>MSQHNEKNPHQHQSPLHDSSEAKPGMDSLAPEDGSHRPAAEPTPPGAQPTAPGSLKAPDTRNEKLNSLEDVRKGSENYALTTNQGVRIADDQNSLRAGSRGPTLLEDFILREKITHFDHERIPERIVHARGSAAHGYFQPYKSLSDITKADFLSDPNKITPVFVRFSTVQGGAGSADTVRDIRGFATKFYTEEGIFDLVGNNTPIFFIQDAHKFPDFVHAVKPEPHWAIPQGQSAHDTFWDYVSLQPETLHNVMWAMSDRGIPRSYRTMEGFGIHTFRLINAEGKATFVRFHWKPLAGKASLVWDEAQKLTGRDPDFHRRELWEAIEAGDFPEYELGFQLIPEEDEFKFDFDLLDPTKLIPEELVPVQRVGKMVLNRNPDNFFAENEQAAFHPGHIVPGLDFTNDPLLQGRLFSYTDTQISRLGGPNFHEIPINRPTCPYHNFQRDGMHRMGIDTNPANYEPNSINDNWPRETPPGPKRGGFESYQERVEGNKVRERSPSFGEYYSHPRLFWLSQTPFEQRH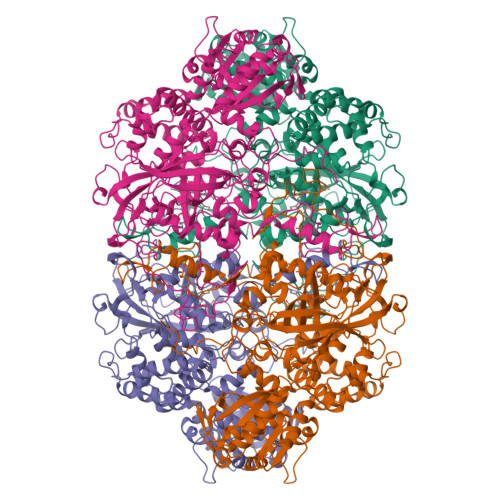IVDGFSFALSKVVRPYIRERVVDQLAHIDLTLAQAVAKNLGIELTDDQLNITPPPDVNGLKKDPSLSLYAIPDGDVKGRVVAILLNDEVRSADLLAILKALKAKGVHAKLLYSRMGEVTADDGTVLPIAATFAGAPSLTVDAVIVPCGNIADIADNGDANYYLMEAYKHLKPIALAGDARKFKATIKIADQGEEGIVEADSADGSFMDELLTLMAAHRVWSRIPKIDKIPA[4x]5-(3-ethylsulfanylphenyl)thiophene-2-carboxamide | C13 H13 N O S2 | 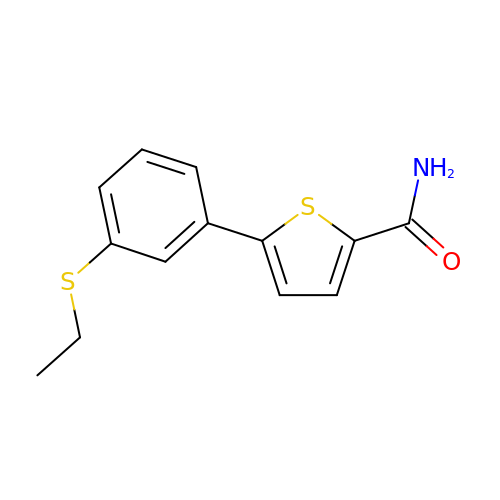TYROLWYYLFWJEG-UHFFFAOYSA-N Here, we report three Pb2+-complexed structures of the thrombin binding aptamer (TBA). These high-resolution crystal structures showed that TBA forms intramolecular G-quadruplex and Pb2+ is bound by the two G-tetrads in the center. Each TBA molecule folds into an antiparallel chair-like quadruplex, which can be divided into four regions: two TT linkers (T3T4 and T12T13), one TGT linker (T7G8T9) and the central G-tetrads. The Pb2+ ion resides in-between the two G-tetrads, coordinating with the eight O6 atoms of the G-tetrads.

In combination with mutagenesis and CD spectra, the G8C mutant structure unraveled that the T7G8T9 linker of TBA is also variable. Substitution of G8 by C8 (for the G8C mutant) or T8 (for the G8T mutant) has no obvious impact on Pb2+-binding; whereas A8 substitution (for the G8A mutant) could lead to stronger Pb2+-binding. Similar to native TBA, we also carried out crystallographic studies for the T7G8T9 linker mutants and successfully solved one complex structure of G8C-Pb2+ at 2.1 Å resolution. The structure belongs to the monoclinic space group C2 and it contains five G8C-Pb2+ complexes per asymmetric unit. Four of the complexes formed two intermolecular dimers, whereas the last one formed dimer with symmetric-related molecule. Other than the A-form structure, the overall folding and orientation of the G8C dimers are more similar to dimer EF in the B-form structure. Due to their different cell units and space groups, packing of G8C-Pb2+ complexes is very different from the A-form and B-form structures. However, the Pb2+-coordinating geometry is almost identical in the three complex structures. C8 is well ordered in the G8C-Pb2+ complex structure. Similar to G8 in the A- and B-form structures, the sugar pucker of C8 also forms stable O–π interaction with G6, which may lead to the similar CD spectra of G8C mutant and native TBA.

>GGTTGGTCTGGTTGG[5x]> GDPVEDIIHDALGNTARRAISSATNVESAANTTPSSHRLETGRVPALQAAETGATSNATDENMIETRCVVNRNGVLETTINHFFSRSGLVGVVNLTDGGTDTTGYATWDIDIMGFVQLRRKCEMFTYMRFNAEFTF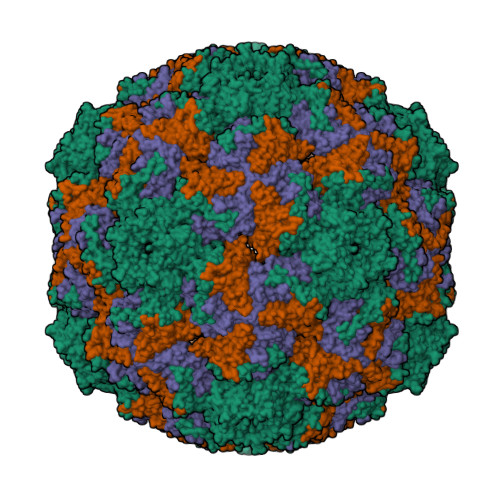VTTTENGGARPYMLQYMYVPPGAPKPTGRDAFQWQTATNPSVFVKLTDPPAQVSVPFMSPASAYQWFYDGYPTFGQHPETSNTTYGLCPNNMMGTFAVRVVSREASQLKLQTRVYMKLKHVRAWVPRPIRSQPYLLKNFPNYDSSKITNSARDRSSIKQANM;> SPSVEACGYSDRVAQLTVGNSSITTQEAANIVLAYGEWPEYCPDTDATAVDKPTRPDVSVNRFYTLDSKMWQENSTGWYWKFPDVLNKTGVFGQNAQFHYLYRSGFCLHVQCNASKFHQGALLVAVIPEFVIAGRGSNTKPNEAPHPGFTTTFPGTTGATFYDPYVLDSGVPLSQALIYPHQWINLRTNNCATVIVPYINAVPFDSAINHSNFGLIVIPVSPLKYSSGATTAIPITITIAPLNSEFGGLRQAVSQ;> GIPAELRPGTNQFLTTDDGTAAPILPGFTPTPTIHIPGEVHSLLELCRVETILEVNNTTEATGLTRLLIPVSSQNKADELCAAFMVDPGRIGPWQSTLVGQICRYYTQWSGSLKVTFMFTGSFMATGKMLVAYSPPGSAQPANRETAMLGTHVIWDFGLQSSVSLVIPWISNTHFRTAKTGGNYDYYTAGVVTLWYQTNYVVPPETPGEAYIIAMGAAQDNFTLKICKDTDEVTQQAVLQ>MESLTQYIPD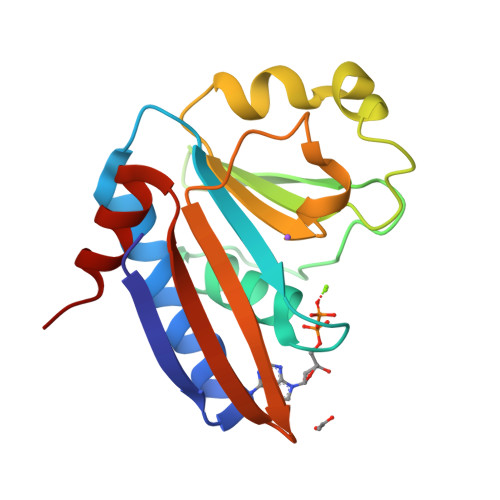EFSMLRFGKKFAEILLKLHTEKAIMVYLNGDLGAGKTTLTRGMLQGIGHQGNVKSPTYTLVEEYNIAGKMIYHFDLYRLADPEELEFMGIRDYFNTDSICLIEWSEKGQGILPEADILVNIDYYDDARNIELIAQTNLGKNIISAFSN[3x]>GSHMDVKAEVIEIIDELFMEDVSDMMDEDLFDAGVLDSMGTVELIVELESRFDIRVPVSEFGRDDWNTANKIVEGVTELRNA[3x];>[4x]MIDFLKQLPHLEPYGNPFYFIYLGIALLPIFIGLFFKKRFAIYECLVSITFIVLALTGTHASQILALLFYIVWQIIWVYSYKRYRSQRDNKWVFYLHSFLVVLPLILVKVEPTINGTQSLLNFLGISYLTFRAVGMIIEMRDGVLKEFTLGEFLRFMLFMPTFTSGPIDRFKRFNEDYQSIPNRDELLNMLEQAVKYIMLGFLYKFVLAQIFGSMLLPPLKAQALSQGGIFNLPTLGVMYVYGFDLFFDFAGYSMFALAVSNLMG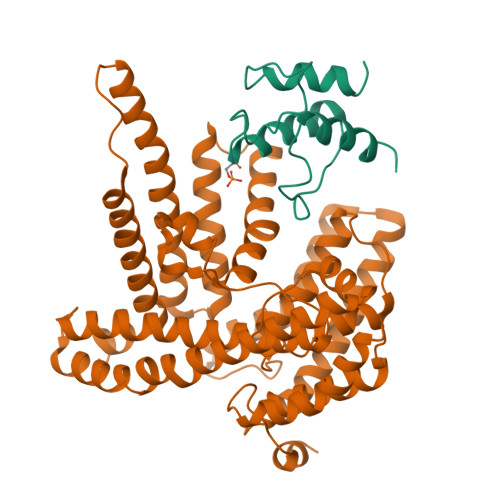IKSPINFDKPFISRDMKEFWNRWHMSLSFWFRDFVFMRLVIVLMRNKVFKNRNTTSNVAYIINMMVMGFWHGITWYYIAYGIFHGIGLVINDAWLRKKKTINKDRKKAGLKPLPENKWTKALGIFITFNTVMLSFLIFSGFLNDLWFTKKLEHHHHHHHH2-(3,4-dihydroxyphenyl)-5,7-dihydroxy-4H-chromen-4-one | C15 H10 O6 | 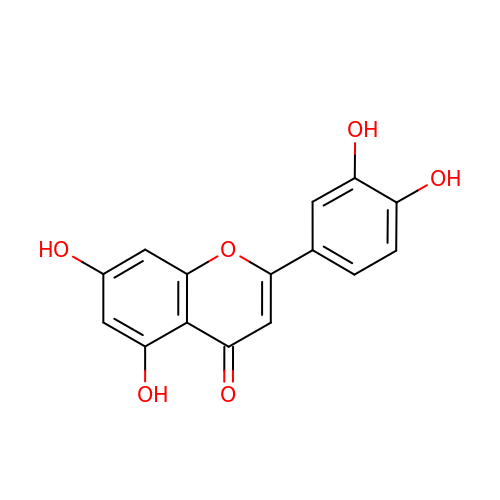IQPNAANSBPBGFQ-UHFFFAOYSA-N>[4x]MAKVQVNNVVVLDNPSPFYNPFQFEITFECIEDLSEDLEWKIIYVGSAESEEYDQVLDSVLVGPVPAGRHMFVFQADAPNPGLIPDADAVGVTVVLITCTYRGQEFIRVG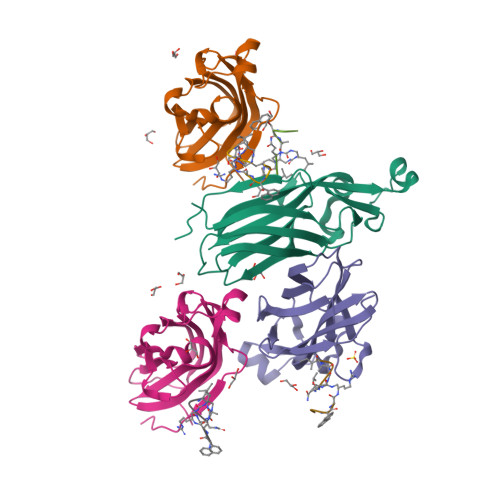YYVNNEYTETELRENPPVKPDFSKLQRNILASNPRVTRFHINWEDN> TITLEKKVRKGIESLITELKLMQAVLSKVSKVPADQLDEGVKIWAGNVKELSYQMEDIVDAFMVRVGDGGESTNPKNRVKKILKKVKKLFKNGKDLHRISAALEEVVLQAKQLAELRQRYEQEMRDTSAQTSVDPRMMALYTDVTELVGIEETRDKLINMLTEGDDWSKHPLKTISIVGFGGLGKTTLAKAAYDKIKVQFDCGAFVSVSRNPEMKKVLKDILYGLDKVKYENIHNAARDEKYLIDDIIEFLNDKRYLIVIDDIWNEKAWELIKCAFSKKSPGSRLITTTRNVSVSEACCSSEDDIYRMEPLSNDVSR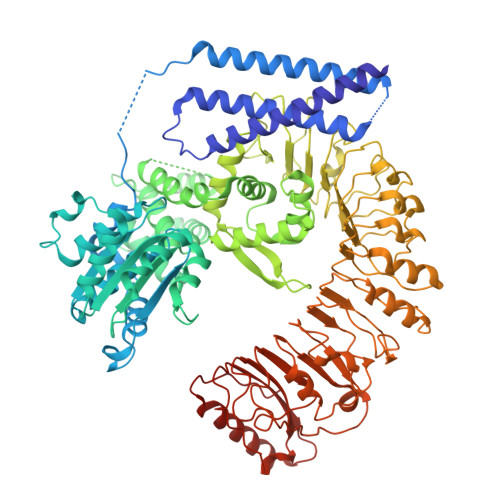TLFCKRIFSQEEGCPQELLKVSEEILKKCGGVPLAIITIASLLANKGHIKAKDEWYALLSSIGHGLTKNRSLEQMKKILLFSYYDLPSYLKPCLLYLSIFPEDREIRRARLVWRWISEGFVYSEKQDISLYELGDSYFNELVNRSMIQPIGIDDEGKVKACRVHDMVLDLICSLSSEENFVTILDDPRRKMPNSESKVRRLSIQNSKIDVDTTRMEHMRSVTVFSDNVVGKVLDISRFKVLRVLDLEGCHVSDVGYVGNLLHLRYLGLKGTHVKDLPMEVGKLQFLLTLDLRGTKIEVLPWSVVQLRRLMCLYVDYGMKLPSGIGNLTFLEVLDDLGLSDVDLDFVKELGRLTKLRVLRLDFHGFDQSMGKALEESISNMYKLDSLDVFVNRGLINCLSEHWVPPPRLCRLAFPSKRSWFKTLPSWINPSSLPLLSYLDITLFEVRSEDIQLLGTLPALVYLEIWNYSVFEEAHEVEAPVLSSGAALFPCATECRFIGIGAVPSMFPQGAAPRLKRLWFTFPAKWSSSENIGLGMRHLPSLQRVVVDVISEGASREEADEAEAALRAAAEDHPNRPILDIW>MLDRFATKQTQEKLKIGVVGTFAIGCLFPLLSDFKRSYPHIDLHISTHNNRVDPAAEGLDYTIRYGGGAWHDTDAQYLCSALMSPLCSPTLASQIQTPADILKFPLLRSYRRDEWALWMQTVGEAPPSPTHNVMVFDSSVTMLEA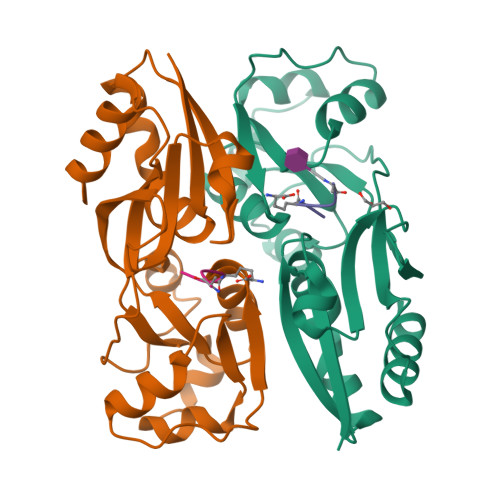AQAGMGVAIAPVRMFTHLLSSERIVQPFLTQIDLGSYWITRLQSRPETPAMREFSRWLTGVLHKTSGSHHHHHH[8x];>[8x]AEKAA> GSDEKRLHFGNGHLKLPGLRTFVDPHTFEDPTQTVHEFAKELDATNISIDKVVGAGEFGEVCSGRLKLPSKKEISVAIKTLKVGYTEKQRR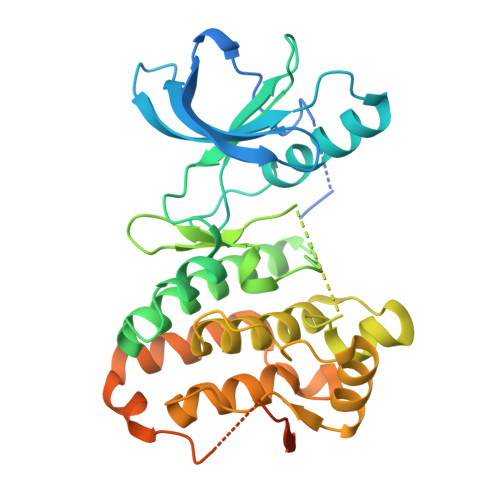DFLGEASIMGQFDHPNIIRLEGVVTKSKPVMIVTEYMENGSLDSFLRKHDAQFTVIQLVGMLRGIASGMKYLSDMGYVHRDLAARNILINSNLVCKVSDFGLGRVLEDDPEAAYTTRGGKIPIRWTSPEAIAYRKFTSASDVWSYGIVLWEVMSYGERPYWEMSNQDVIKAVDEGYRLPPPMDCPAALYQLMLDCWQKDRNNRPKFEQIVSILDKLIRNPGSLKIITSAAARPSNLLLDQSNVDITTFRTTGDWLNGVWTAHCKEIFTGVEYSSCDTIAKIS>[2x]SVIEKLRKLEKQARKQGDEV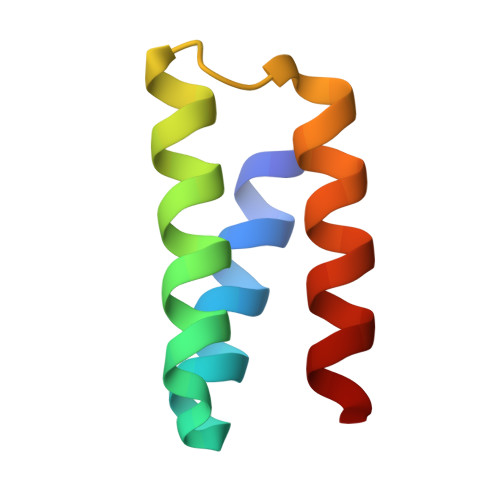LVMLARMVLEYLEKGWVSEEDADESADRIEEVLKK>[4x]MSLASLIGLAVCTGNAFSPALAAEAKQPNLVIIMADDLGYGDLATYGHQIVKTPNIDRLAQEGVKFTDYYAPAPLSSPSRAGLLTGRMPFRTGIRSWIPSGKDVALGRNELTIANLLKAQGYDTAMMGKLHLNAGGDRTDQPQAQDMGFDYSLANTAGFVTDATLDNAKERPRYGMVYPTGWLRNGQPT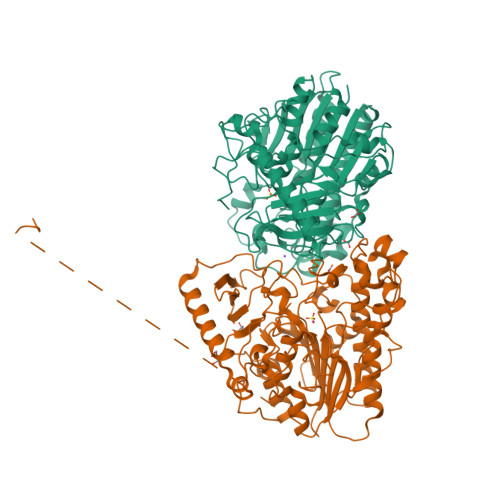PRADKMSGEYVSSEVVNWLDNKKDSKPFFLYVAFTEVHSPLASPKKYLDMYSQYMSAYQKQHPDLFYGDWADKPWRGVGEYYANISYLDAQVGKVLDKIKAMGEEDNTIVIFTSDNGPVTREARKVYELNLAGETDGLRGRKDNLWEGGIRVPAIIKYGKHLPQGMVSDTPVYGLDWMPTLAKMMNFKLPTDRTFDGESLVPVLEQKALKREKPLIFGIDMPFQDDPTDEWAIRDGDWKMIIDRNNKPKYLYNLKSDRYETLNLIGKKPDIEKQMYGKFLKYKTDIDNDSLMKARGDKPEAVTWGEGHHHHHH4-[(2-methoxypyridin-3-yl)sulfamoyl]benzene-1-sulfonic acid 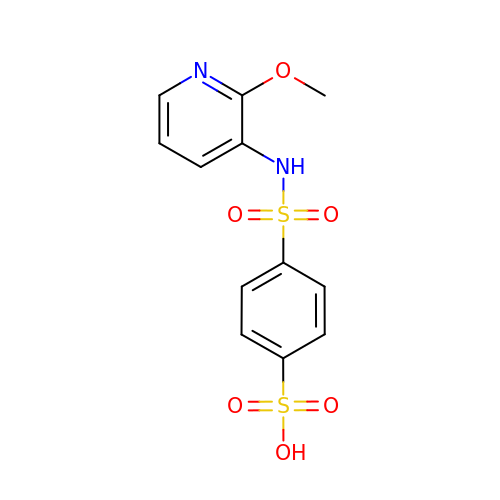| C12 H12 N2 O6 S2 | YXYLOWSJBFRQDN-UHFFFAOYSA-N1-(2-azaspiro[5.6]dodecan-2-yl)ethan-1-one 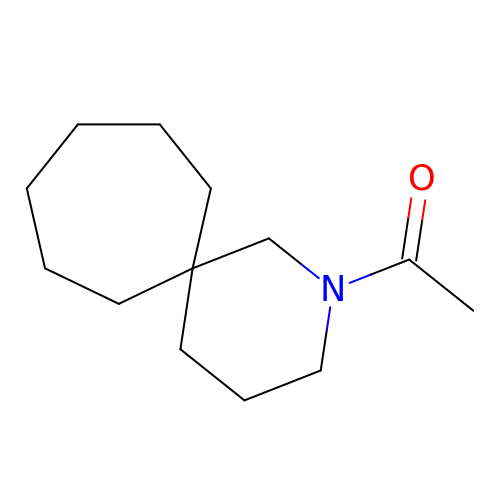| C13 H23 N O | JPZFTAQMOATKEN-UHFFFAOYSA-N>MKDGMRVGERFTHDFVVPPHKTVRHLYPESPEFAEFPEVFATGFM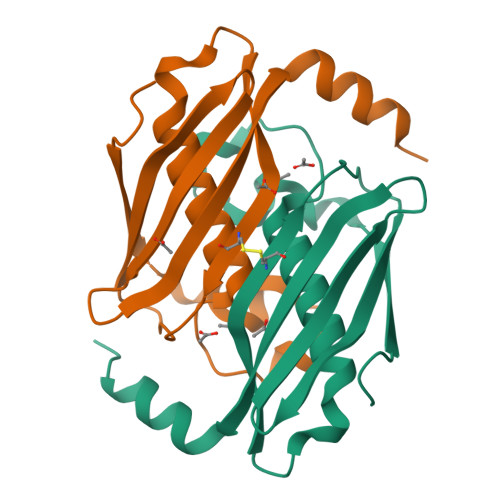VGLMEWACVRAMAPYLEPGEGSLGTAICVTHTAATPPGLTVTVTAELRSVEGRRLSWRVSAHDGVDEIGSGTHERAVIHLEKFNAKVRQKTPAG[2x]In the NRC immune receptor network of solanaceous plants, multiple sensor CC-NLRs can signal redundantly via an array of downstream paralogous helper CC-NLRs termed NRCs (NLRs required for cell death) to confer disease resistance to a multitude of pathogens and pests. Here, we show that the coiled-coil helper NLR NRC2 from Nicotiana benthamiana accumulates in vivo as a homodimer that converts into a higher-order oligomer upon activation by its upstream virus disease resistance protein Rx. We show that unlike the canonical CC-NLR AtZAR1, NbNRC2 forms a homodimer in its resting state. Mutagenesis of various residues in the NbNRC2 homodimerization interface led to impaired self-association and effector-independent activation, suggesting that homodimerization contributes to immune receptor autoinhibition.

To further investigate the resting form of NbNRC2, we transiently expressed and affinity-purified NbNRC2 from leaves of N. benthamiana. Cryo-EM imaging of these particles and single particle reconstruction revealed a homodimer structure at a resolution range of 3.9 to 4.5 Å with C2 symmetry imposed. The reconstructed structure contains the NB-ARC and LRR domains of NbNRC2, with the N-terminal CC domain appearing disordered in the density map. Flexible fitting of the AlphaFold2 model of NbNRC2 monomers into the cryo-EM map of the dimeric assembly revealed the relative orientation of the helper NLR protomers as well as the domains responsible for homodimer organisation. The NB domain of each NbNRC2 protomer interacts with the LRR region of the other protomer, forming 2 similar interfaces related by 2-fold symmetry of the dimer (interface 1 and interface 3). The N-terminal LRR region of each NbNRC2 protomer stacks over the equivalent region of the other protomer, at the 2-fold symmetry, forming interface 2. These 3 interfaces hold the homodimer together with a buried surface area 937 Å2 for each protomer, making the total buried surface 1874 Å2. Interfaces 1 and 3 are composed of 3 stretches of residues in the NB domain (Stretch 1a-1c, residues 217–220, 238–244, and 270–274, respectively) in 1 protomer and 3 stretches of residues in the LRR (stretches 1d-1f, residues 506–513, 533–536, and 559–563, respectively) from the other protomer. Two stretches of residues in the LRR (stretches 2a and 2b, residues 528–532 and 549–554, respectively) stack together forming interface 2. The surfaces involved in NbNRC2 homodimerization are surface exposed in the activated NbNRC2 hexamer structure.

>[2x]MANVAVEFLVQNLMQLLRDNAELIVGVKDSAESLLQDLNDFNAFLKQTAKSRTENDVHKELVKKIKTVVNSAEDAIDKFVIEAKLHKDKGVGRFVDVKHYKRVYDVAGEIKTIRDKVKEIRLNNALDLQALQDEDQSAKGVQERKPPVVEEDDVVGFEEEADKVINRLLGGSSGLEVVPVVGMPGLGKTTLANKIYKHPDIGYQFFTRIWVYVSQSYRRRELFLNIISKFTRNTKQYHDMCEEDLADEIEDFLGKGGKYLIVLDDVWSPDAWERIRIAFPNNNKSNRILLTTRDSKVAKQCKQCIGIPHDLKFLTEDESWILLEKKVFHKDKCPPELELSGKSIAKKCNGLPLAIVVIAGALIGKGKTSREWKQVDESVGEHLINKDQPENCNKLVQLSYDRLSYDLKACFLYCGAFPGGFEIPAWKLIRLWIAEGFIQYKGHLSLECKAEDNLNDLINRNLVMVMQRTSDGQIKTCRLHDMLHEFCRQEAMKEENLFQEIKLGAEQYFPGKRELATYRRLCIHSSVLEFISTKPSGEHVRSFLSFSLKKIEMPSVDIPTIPKGFPLLRVFDVESINFSRFSKEFFQLYHLRYIAFSSDTIKIIPKHIGELWNIQTLIINTQQRSLDIQANIWNMERLRHLHTNSSAKLPVPVTPRSSKVPLVNQSLQTLSTIAPESCTEEVFARTPNLKKLGIRGKIAVLLEPNKSLLKNVKKLESLENLKLINDSSQTGKGLRLPPSYIFPTKLRKLSLVDTWLEWNDMSILGQMEHLEVLKLKENGFMGECWESVGGFCSLLVLWIERTDLVSWKASADHFPRLKHLVLICCDKLKEIPIGLADIRSFQVMELQNSTKTAAISARGIRDKKDKQTQEGTNNNGFKLSIFPPDLGSGSGRGSHHHHHHDYDIPTTASENLYFQGELDYKDHDGDYKDHDIDYKDDDDK> GPGSDNEALLRRQFPIFHWSAANKVVYAVPPIPDQSQYMISSSIVQEIKVTPIDQIIKPNDMLKSFPGPLGSAKLKKKDLTKWMETTIKSISENESSTDMTIWQLLEMKLNDKVNWKNISKLLYNSDELLMYLSQ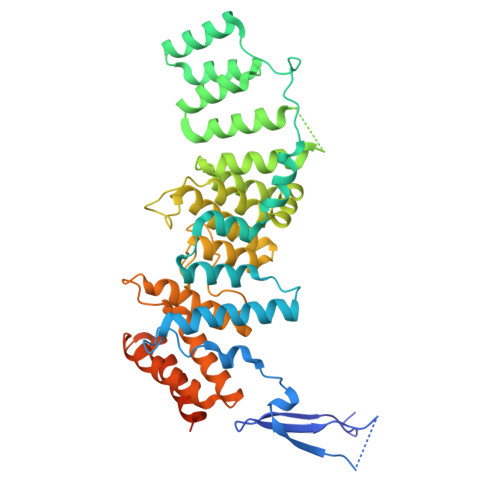PFPNGDMIPNAYRLDINCQMRVLAFLQTGNHDEALRLALSKRDYAIALLVGSLMGKDRWSEVIQKYLYEGFTAGPNDQKELAHFLLLIFQVFVGNSKMAIKSFYTNNETSQWASENWKSIVAAVLINIPENNEDPLLIPPVVLEFLIEFGIFLTKKGLTAAASTLFIIGNVPLSNEPVMADSDVIFESIGNMNTFESILWDEIYEYIFSYDPKFKGFSSILPQKIYHASLLQEQGLNSLGTKYTDYLSSSVRKLPKKDILTINLTRELSEVASRLSESNTGWLAKPKLSSVWGQLDKSFNKYIGGD>MGNIMSASFAPECTDLKTKYDSCFNEWYSEKFLKGKSVENECSKQWYAYTTCVNAALVKQGIKPALDEAREEAPFENGGKL[8x];>MGSSHHHHHHSQDPMVLLHKSTHIFPTDFASVSRAFFNRYPNPYSPHVLSIDTISRNVDQEGNLR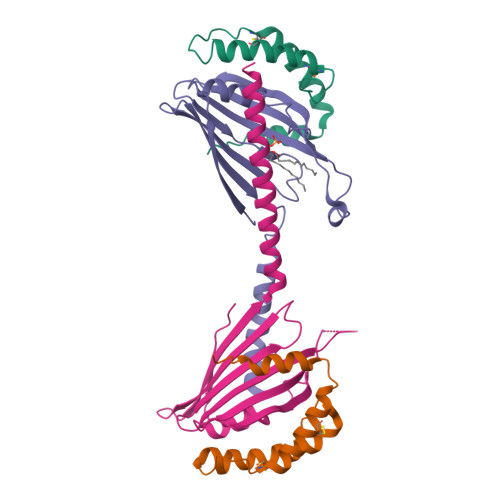TTRLLKKSGKLPTWVKPFLRGITETWIIEVSVVNPANSTMKTYTRNLDHTGIMKVEEYTTYQFDSATSSTIADSRVKFSSGFNMGIKSKVEDWSRTKFDENVKKSRMGMAFVIQKLEEA[8x]> MYQLEKEPIVGAETFYVDGAANRETKLGKAGYVTNRGRQKVVTLTDTTNQKTELQAIY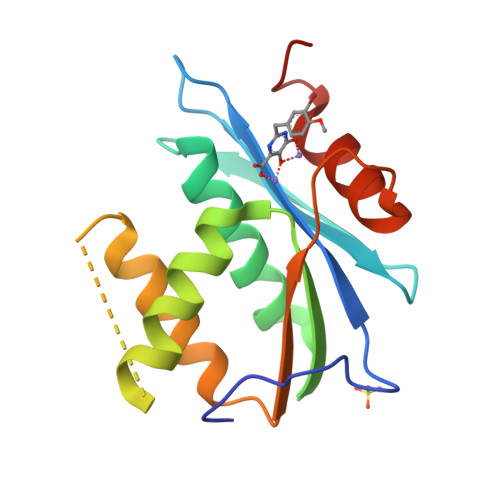LALQDSGLEVNIVTDSQYALGIITQWIHNWKKRGWKTADKKPVKNVDLVNQIIEQLIKKEKVYLAWVPAHKGIGGNEQVDKLVSAGIRKVLF> MAADRDNFLQNIENDSINNGQAMDLSPNRSSSESDSSILMNVNDIKTLRLDVAPEAKSTQSKKSLFYENSDDAEEGEIEERTNKEEGQYHHKGSKQLRFEVGKESTGKLQSHLSDGSATSGEGNVRPWEFRKVIQAEYRERLPRNYELKHWKKPSKIMIGSILRLLETNTVSALDSVFEKYEKEMNQMTHGDNNEVKRIYSKKERLLEIILTKIKKKLRQAKFPSRISERDLDIEYIYSKRQFIQNRYSQELQNNERLEAILSREQNLLEETRKLCMNLKTNNKKRLTEKLIQKDLHPVLNKAMEYTYGLESTNGFMHPDGPVTFRNDSHELNLMLNDPIKSTADVRLDKE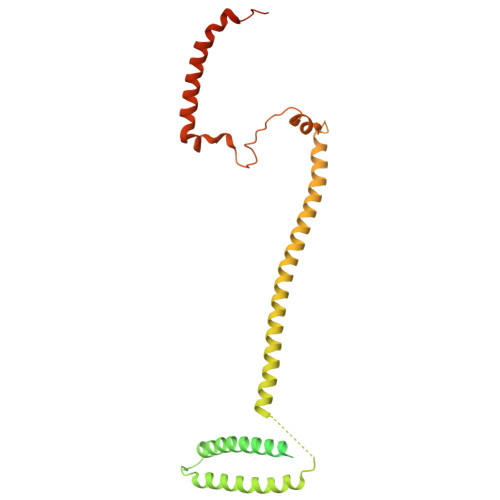EVLSLLPSLKEYTKKSKELKETMGQMISDSHEEEIKEVFVPHHESHQDKTEEDIH>[4x]GSARDISSTNVTDLTVSPSKIEDGGKTTVKMTFDDKNGKIQNGDMIKVAWPTSGTVKIEGYSKTVPLTVKGEQVGQAVITPDGATITFNDKVEKLSDVSGFAEFEVQGRNLTQTNTSDDKVATITSGNKSTNVTVHKSEAGTSSVFYYKTGDMLPEDTTHVRWFLNINNEKSYVSKDITIKDQIQGGQQL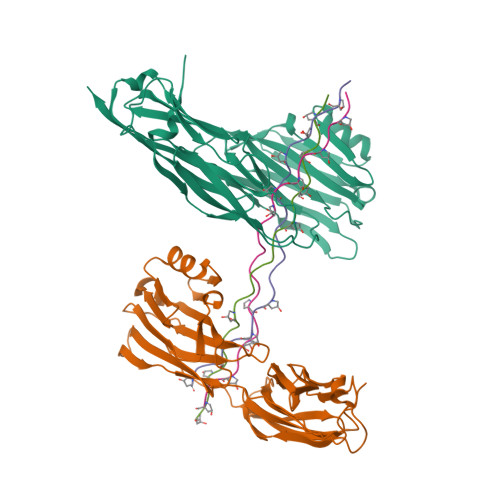DLSTLNINVTGTHSNYYSGQSAITDFEKAFPGSKITVDNTKNTIDVTIPQGYGSYNSFSINYKTKITNEQQKEFVNNSQAWYQEHGKEEVNGKSFNHTVHNINANAGIEGTVK;>[6x]GPPGPPGPPGPPGPRGRTGPPGPPGPPGPP>MNNVEKAIEALKKGEIILVYDSDEREGETDMVVASQFITPEHIRIMRKDAGGLICTALHPDICNKLGIPFMVDILEFASQKFKVLRELYPNDIPYDEKSSFSITINHRKTFTGITDNDRAFTIKKLAELVKEGRFNDFGKEFRSPGHVTLLRAAEGLVKNRQGHTEMTVALAELANLVPITTI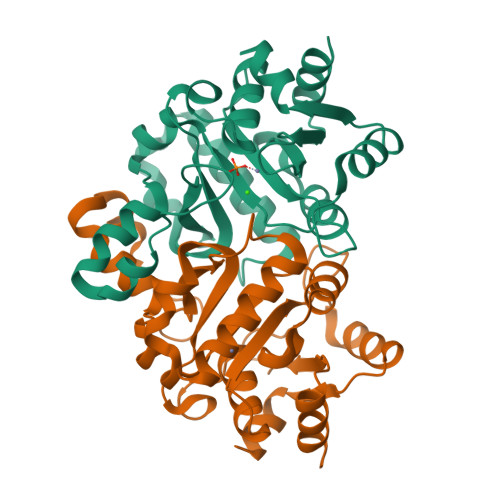CEMMGDDGNAMSKNETKRYAEKHNLIYLSGEEIINYYLDKYLKD[3x]>MSLTADTKRPLTLRDVSEASGVSEMTVSRVLRNRGDVSDATRARVLAAAKELGYVPNKIAGALASNRVNLVAVIIPSLSNMVFPEVLTGINQVLEDTELQPVVGVTDYLPEKEEKVLYEMLSWRPSGVIIAGLEHSEAARAMLDAAGIPVVEIMDSDGKPVDAMVGISHRRAGREMAQAILKAGYRRIGFMGTKMPLDYRARKRFEGFTEVLGKNGVEIEDREFYSGGSALAKGREMTQAMLERSPDLDFLYYSNDMIAAGGLLYLLEQGIDIPGQIGLA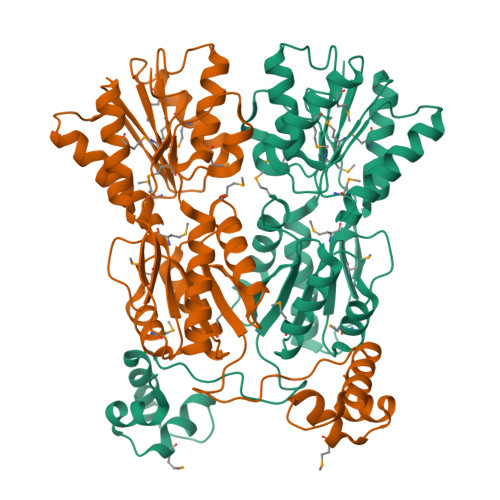GFNNVELLQGLPRKLATMDACRLEIGRKAAEIIAKRLEDPEAEIETRITLEPKISYGDTLKREG[4x]> MMQQSRPASDPQVVEAARKEGRLIIYSSTDQSSAQALLDDFRKLYPFIQIEYNDLGTQAIYDRFVSETAAGASSADLLWSAAMELQVKLASEGYALPYDSPEAKNWPANARLGNLAYSTTLEPAVVVYNKRFLKPEEVPTTREGLARLLQEPRMRGRVATWDPERSAVGFTILKADYDRFPAFQELARAFGKAQAALYSSTGAAFEKVISGEHYLAYGFFGSYALLRQRTVKDLGIAYLTDGTVAIQRVAFINKRAAHPNAAKLFLDYLLSLRGQNLMAYTALIFARRETVVGEATPQALYKAVGGKDKVYAIPVSTEILKNLDPA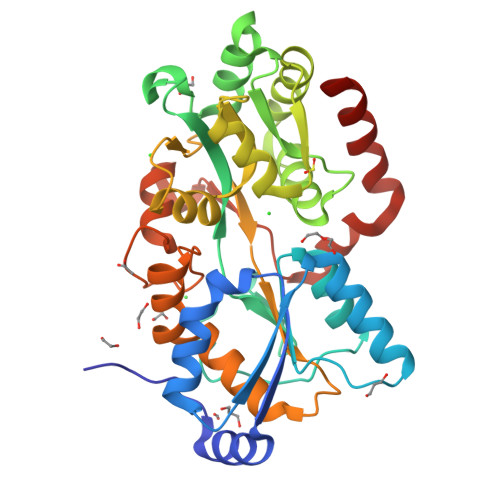ERMRFLTFWRQAVRGQ> LSSNHKEVFKGHNLPRLRGAMIGPHVTNADLLEFGNVWKANHIRWQLIWNGFPHSPADSATLDEYRQWLDGALKRLEAALPVCREAGILVTVDLHTPPGGRNEASECRIFHDR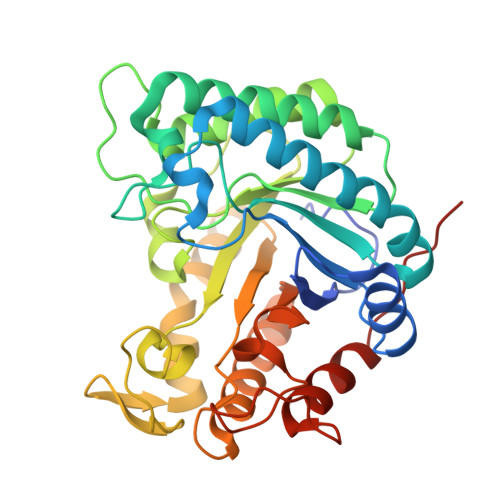EFQKAFIDIWEDIARRFADSDVVWGYDLVNAPVEGMVPDGLMNWQRLAEETARRVRAIDQKHAIIIEPAPWGSPSSIALLDPIDVPGVVYSVHMYVPHAFTHQGVYDNPVGIVYPGTIDGKWYDRNTLRKVLEPVRRFQEENGVHIYIGEFSAIRWAPADSACQYLKDCIEIFEEYGWDWAYHAFREWDGWSVEHGPDRNDRNRTATPTDRALLLRSWYAENVKPQFSDKKKD> IISRNFPIIGVKEKTFEQLHKKCLEKKVLYVDPEFPPDETSL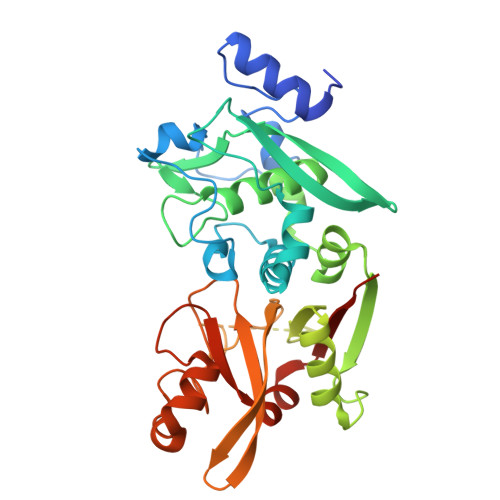FYSQKFPIQFVWKRPPEICENPRFIIDGANRTDICQGELGDCWFLAAIACLTLNQHLLFRVIPHDQSFIENYAGIFHFQFWRYGEWVDVVIDDCLPTYNNQLVFTKSNHRNEFWSALLEKAYAKLHGSYEALKGGNTTEAMEDFTGGVAEFFEIRDAPSDMYKIMKKAIERGSLMGCSIDDGTNMTYGTSPSGLNMGELIARMVRNMDNSLLQDSDLDPRGSDERPTRTIIPVQYETRMACGLVRGHAYSVTGLDEVPFKGEKVKLVRLRNPWGQVEWNGSWSDRWKDWSFVDKDEKARLQHQVTEDGEFWMSYEDFIYHFTKLEICNLTADLEHHHHHH> AHHHHHHGSNKRFPFPVGEPDFIQGDEAIARAAILAGCRFYAGYPITPASEIFEAMALYMPLVDGVVIQMEDEIASIAAAIGASWAGAKAMTATSGPGFSLMQENIGYAVMTETPV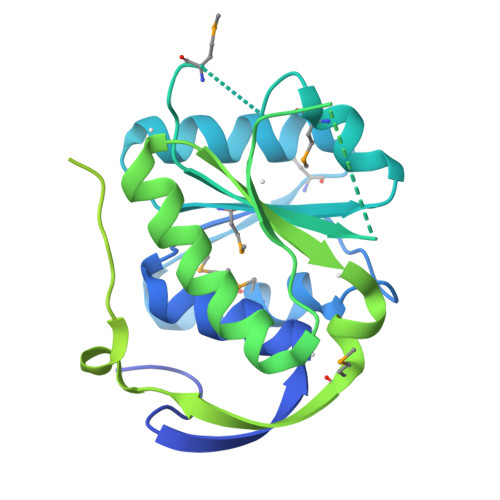VIVDVQRSGPSTGQPTLPAQGDIMQAIWGTHGDHSLIVLSPSTVQEAFDFTIRAFNLSEKYRTPVILLTDAEVGHMRERVYIPNPDEIEIINRKLPRNEEEAKLPFGDPHGDGVPPMPIFGKGYRTYVTGLTHDEKGRPRTVDREVHERLIKRIVEKIEKNKKDIFTYETYELEDAEIGVVATGIVARSALRAVKMLREEGIKAGLLKIETIWPFDFELIERIAERVDKLYVPEMNLGQLYHLIKEGANGKAEVKLISKIGGEVHTPMEIFEFIRREFK>[2x]MGGSHHHHHHGTMKQLISLKNIFRSYRNGDQELQVLKNINLEVNEGEFVAIMGPSGSGKSTLMNTIGMLDTPTSGEYYLEGQE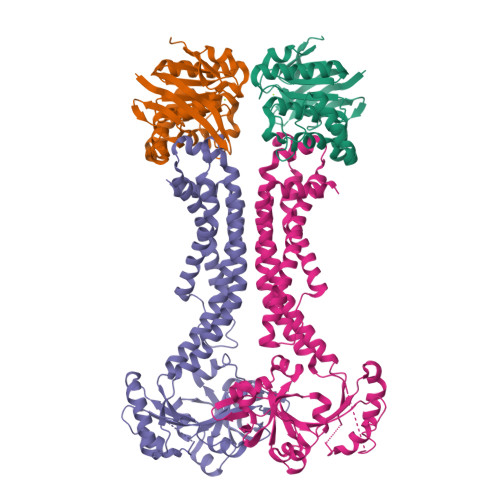VAGLGEKQLAKVRNQQIGFVFQQFFLLSKLNALQNVELPLIYAGVSSSKRRKLAEEYLDKVELTERSHHLPSELSGGQKQRVAIARALVNNPSIILADEPTGALDTKTGNQIMQLLVDLNKEGKTIIMVTHEPEIAAYAKRQIVIRDGVISSDSAQLGKEEN;>[2x]MQNLKFAFSSIMAHKMRSLLTMIGIIIGVSSVVVIMALGDSLSRQVNKDMTKSQKNISVFFSPKKSKDGSFTQKQSAFTVSGKEEEVPVEPPKPQESWVQEAAKLKGVDSYYVTNSTNAILTYQDKKVENANLTGGNRTYMDAVKNEIIAGRSLREQDFKEFASVILLDEELSISLFESPQEAINKVVEVNGFSYRVIGVYTSPEAKRSKIYGFGGLPITTNISLAANFNIDEIASIVFRVNDTSLTPTLGPELARKMTELAGLQQGEYQVADESVVFAEIQQSFSFMTTIISSIAGISLFVGGTGVMNIMLVSVTERTREIGLRKALGATRANILIQFLIESMILTLLGGLIGLTIASGLTALAGLLLQGLIEGIEVGVSIPVALFSLAVSASVGMIFGVLPANKASKLDPIEALRYE> MEDINFASLAPRHGSRPFMGNWQDIGTSNMSGGAFSWGSLWSGIKNFGSTVKNYGSKAWNSSTGQMLRDKLKEQNFQQKVVDGLASGISGVV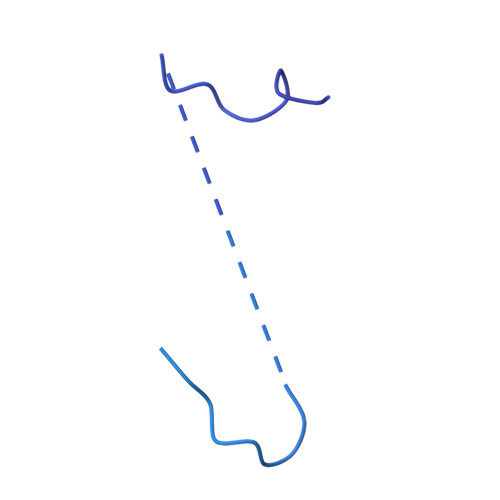DLANQAVQNKINSKLDPRPPVEEPPPAVETVSPEGRGEKRPRPDREETLVTQIDEPPSYEEALKQGLPTTRPIAPMATGVLGQHTPVTLDLPPPADTQQKPVLPGPTAVVVTRPSRASLRRAASGPRSLRPVASGNWQSTLNSIVGLGVQSLKRRRCF> NGDRLYRADSRPPDEIKRSGGLMPRGHNEYFDRGTQMNINLYDHARGTQTGFVRYDDGYVSTSLSLRSAHLAGQSILSGYSTYYIYVIATAPNMFNVNDVLGVYSPHPYEQEVSALGGIPYSQIYGWY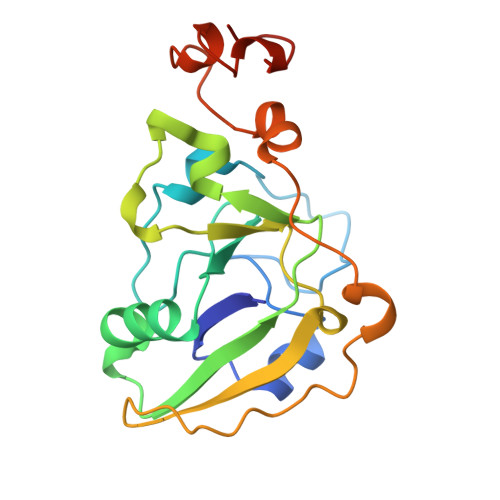RVNFGVIDERLHRNREYRDRYYRNLNIAPAEDGYRLAGFPPDHQAWREEPWIHHAPQGCGNSSR Clostridium acetobutylicum ATCC 824 gene CA_C0359 encodes a putative unsaturated rhamnogalacturonyl hydrolase (URH) with distant amino-acid sequence homology to YteR of Bacillus subtilis strain 168. GH105 proteins have been shown to cleave plant-based and algae-based substrates by hydrolyzing small two-chain and three-chain unsaturated polysaccharides containing an unsaturated uronyl saccharide at the non­reducing end. The suggested mechanism for both families requires hydration at the C=C bond of the unsaturated sugar, resulting in glycosidic cleavage. Transcriptional studies and structural analysis of the CA_C0359-derived protein product presented here support its annotation as a GH105 family protein with an active pocket capable of binding unsaturated polysaccharides containing an unsaturated galacturonate.

Crystals of the CA_C0359 protein belonged to space group P212121, with two molecules in the asymmetric unit and a solvent content of approximately 47.6%, as determined using the Matthews coefficient. The protein adopts a six-(α/α)-hairpin barrel fold with a small two-stranded β-sheet and helix overlaying the end of the barrel near the active pocket. The two tertiary structures align with a root-mean-square deviation of 1.4 Å and contain a highly conserved active pocket. When the sequence alignment was fitted to a surface rendering of the CA_C0359 structure, the putative active-site pocket was highly concentrated with conserved residues. The character of the CA_C0359 active-site pocket is somewhere between that of YteR and UGL. The representative PatchDock results demonstrate that the conserved residues Asp130, His176, Asp75 and Tyr25 are available for binding the three disaccharides of interest. While the mobile loop of CA_C0359 (residues 320–330) may provide some gating action, it is unlikely to completely block access to the active-site pocket. The catalytic site of Cac_GH105 is slightly more open than those of YteR and YesR, and not as open as Nu_GH105, which may allow larger sugars to fit the +1 subsite, and possibly trioligosaccharides and tetraoligosaccharides. Conversely, the loop extending from the gate loop of Cac_GH105, which is not observed in the other GH105 structures, may play an important role in substrate specificity compared with other proteins in this family. Taken with the electrostatic comparison and growth on pectin and PGA, Cac_GH105 may cleave a wider range of substrates than or a different range of substrates to YteR, including ΔGalA-Rha and ΔGalA-GalA, which may be decorated with side chains or be longer-chained oligosaccharides.

>MQKYSKLMADSIIAKNITLTDHWGYEYGLTLDGIAKVYEWTKDKKYLDFIIKTMDTFINEDGTINGYKLEEYNIDHLNNGKILITLFKETGKEKYRKALINLRKQIDNHPRTKENVFWHKNIYPHQIWLDGLYMGATFYAKYVKEFGEEKEFDDITHQFIITEKNLKDNKTGLLYHAYDESKTEPWSNSETGLSPHFWGRAMGWYVMALADTIEVLPKNHKDRNALIKILNNCVTALLKVQDNASKVWYQVLDEGERKGNYLEASGSSMIVYALLKGVRLGYLPESLKETAKEAYKGLINEFILETKDGLINLNKICYVAGLGGKDKRDGSFAYYISEPIVSNEPKGLGPFLLASYEYETL[2x]>MFGKGGLGNLMKQAQQMQEKMQKMQEEIAQLEVTGESGAGLVKVTINGAHNCRRVEIDPSLLED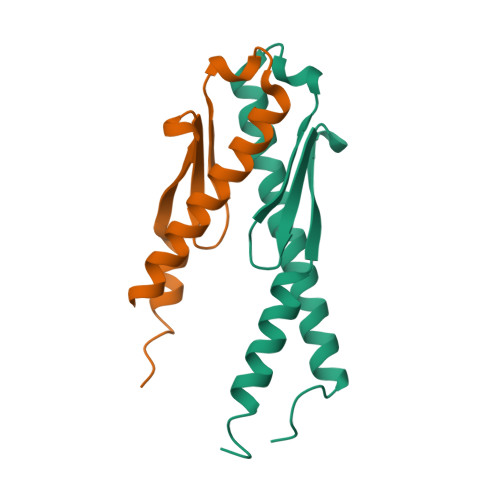DKEMLEDLVAAAFNDAARRIEETQKEKMASVSSGMQLPPGFKMPF[4x]> TVKIWVKYNEGF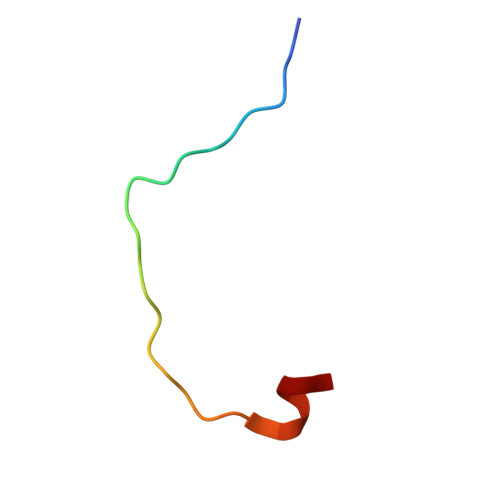SNAVRKNVTWNNLW> GPPGPKGDPGPKGDPGPPGARGQAGVL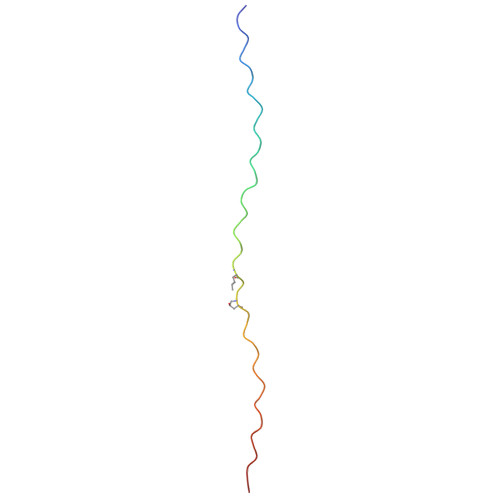GFPGPPGPPGPKGDKGDPGGYX>[4x]GSGLSKPYMDVVGFAKTESEFETRETHGELNLNSVPIYNGELDFSDKIMKRSSTKVIGTLEELLENSPCSALEGISKWHKIGGSVKDGVLCILSQDFLFKALHVLLMSAMAESLDLQHLNVEDTHHAVGKDIEDEFNPYTREIIETV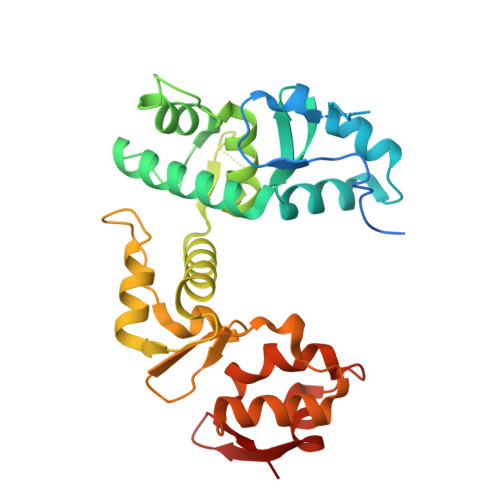LNKFAVQEQEAENNTWRLRIPFIAQWYGIQALRKYVSGISMPIDEFLIKWKSLFPPFFPCDIDIDMLRGYHFKPTDKTVQYIAKSTLPMDPKERFKVLFRLQSQWDLEDIKPLIEELNSRGMKIDSFIMKYARRKRLGKKTVVTSR> GGHMEPLDELDLLLLEEDGGAEAVPRVELLRKKADALFPETVLSRGVDNRYLVLAVETSQNERGAEEKRLHVTASQDREHEVLCILRNGWSSVPVEPGDIVHLEGDCTSEPWIIDDDFGYFILYPDMMISGTSVASSIRCLRRAVLSETFRGSDPATRQMLIGTILHEVFQKAISESFAPERLQELALQTLREVRHLKEMYRLNLSQDEILCEVEEYLPSFSKWAEDFMRKGPSSEFPQMQLSLPSDGSNRSSPCNIEVVKSLDIEESIWSPRFGLKGKIDVTVGVKIHRDCKMKYKVMPLELKTGKESNSIEHRSQVVLYTLLSQERREDPEAGWLLYLKTGQMYPVPANHLDKRELLKLRNWLAASLLHRVSRAAPGEEARLSALPQIIEEEKTCKYCSQIGNCALYSRAVEEQGDDASIPEAMLSKIQEETRHLQLAHLKYFSLWCLMLTLESQSKDNRKTHQSIWLTPASELEESGNCVGNLVRTEPVSRVCDGQYLHNFQRKNGPMPATNLMAGDRIILSGEERKLFALSKGYVKKMNKAAVTCLLDRNLSTLPATTVFRLDREERHGDISTPLGNLSKLMESTDPSKRLRELIIDFREPQFIAYLSSVLPHDA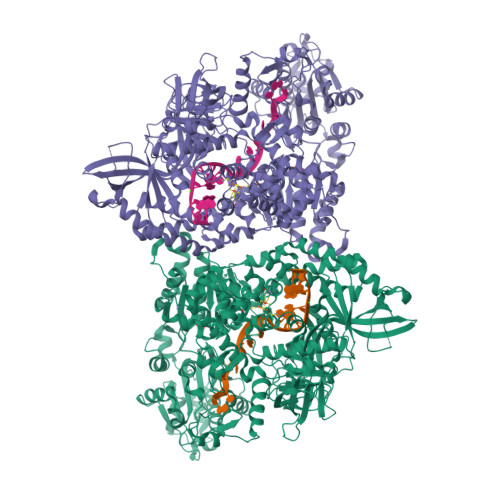KDTVANILKGLNKPQRQAMKRVLLSKDYTLIVGMPGTGKTTTICALVRILSACGFSVLLTSYTHSAVDNILLKLAKFKVGFLRLGQSHKVHPDIQKFTEEEICRSRSIASLAHLEELYNSHPIVATTCMGINHPIFSRKTFDFCIVDEASQISQPVCLGPLFFSRRFVLVGDHQQLPPLVVNREARALGMSESLFKRLERNESAVVQLTVQYRMNRKIMSLSNKLTYAGKLECGSDRVANAVLALPNLKDARLSLQLYADYSDSPWLAGVLEPDNPVCFLNTDKVPAPEQVENGGVSNVTEARLIVFLTSTFIKAGCSPSDIGVIAPYRQQLRIISDLLARSSVGMVEVNTVDKYQGRDKSLILVSFVRSNEDGTLGELLKDWRRLNVALTRAKHKLILLGSVSSLKRFPPLGTLFDHLNAEQLILDLPSREHESLSHIL> MKRARPSEDTFNPVYPYDTETGPPTVPFLTPPFVSPNGFQESPPGVLSLRLSEPLVTSNGMLALKMGNGLSLDEAGNLTSQNVTTVSPPLKKTKSNINLEISAPLTVTSEALTVAAAAPLMVAGNTLTMQSQAPLTVHDSKLSIATQGPLTVSEGKLALQTSGPLTTTDSSTLTITASPPLTTATGSLGIDLKEPIYTQNGKLGLKYGAPLHVTDDLNTLTVATGPGVTINNTSLQTKVTGALGFDSQGNMQLNVAGGLRIDSQNRRLILDVSYPFDAQNQLNLRLGQGPLFINSAHNLDINYNKGLYLFTASNNSKKLEVNL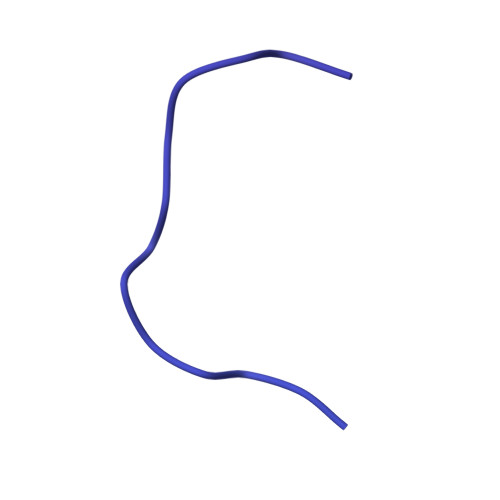STAKGLMFDATAIAINAGDGLEFGSLNAPNSNPLKTKIGHGLEFDSNKAMVPKLGTGLSFDSTGAITVGNKNNDKLTLWTTPAPSPNCRLNAEKDAKLTLVLTKCGSQILATVSVLAVKGSLAPISGTVQSAHLIIRFDENGVLLNNSFLDPEYWNFRNGDLTEGTAYTNAVGFMPNLSAYPKSHGKTAKSNIVSQVYLNGDKTKPVTLTITLNGTQETGDTTPSAYSMSFSWDWSGHNYINEIFATSSYTFSYIAQE>NFFQFAEMIVKMTGKEAVHSYAIYGCYCGWGGQGKPQDATDRCCFVHDCCYGTVNDCNPKMATYSYSFENGDIVCGDNNLCLKTVCECDRAAAICLGQNVNTYDKNYENYAISHCTEESEQC[4x];>NLFQFARLIDAKQEAFSFFKYISYGCYCGWG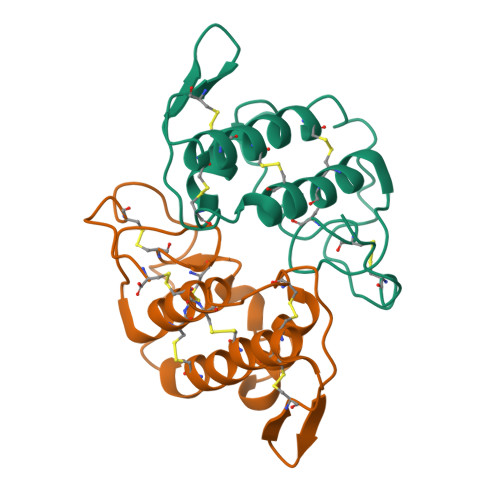GQGTPKDATDRCCFVHDCCYARVKGCNPKLVEYSYSYRTGKIVCGGDDPCLRAVCECDRVAAICFRENMNTYDKKYMLYSIFDCKEESDQC[4x]>[4x]GAMDTMESIVLNTIVTGLQEPKKEFIARVIKTIGSQRSLQLYENAMKVENSGGL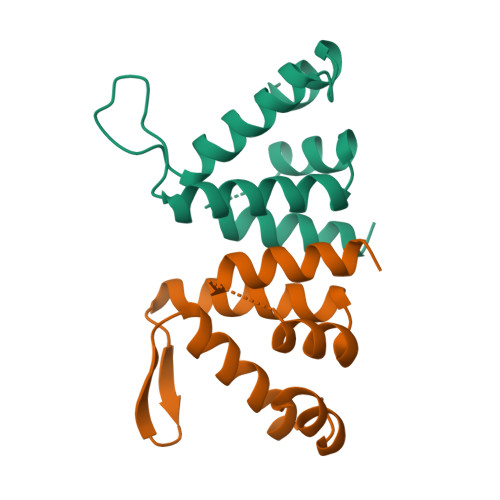LTADMSRRKTIGGVFCYLLKQLVAEDQITIQEWNYIRQEEKERINAKNILKRNNRRCQV>GPPGPPGPPGVPGEAGPPGPPG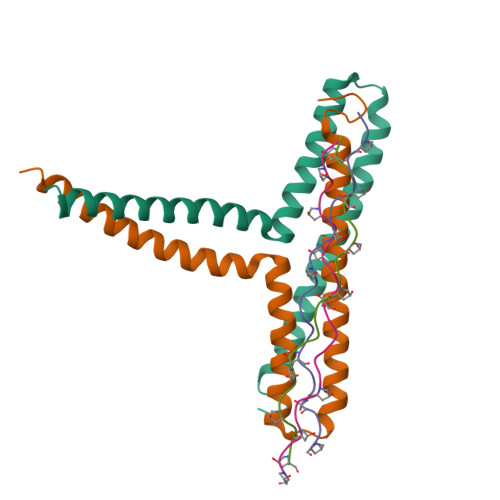PP[6x];>[4x]GAMDARSVNGEFPRHVKLKNEIENLLDQVTQLYTKHNSNYQQYNAQAGRLDLRQKAEYLKGLNDWAERLLQELNGEDVKKVLGKVAFEKDDLEKEVKELKEKIDKKEKEYQDC> LFRAL;> AKCVSYGVAQIKAPALHSQGYTGSNVKVAILGTGIDSSHPDLNVAG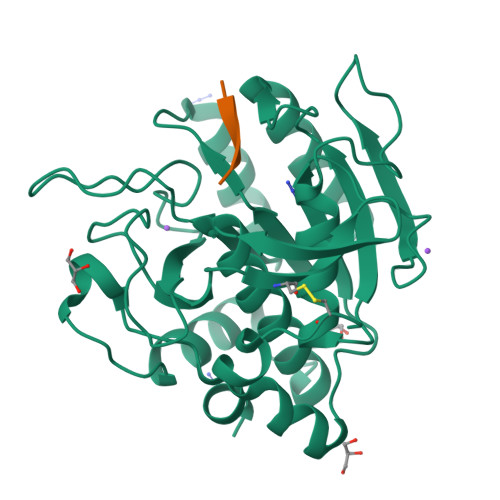GASFVPSETNPFQDNSSHGTHIAGTVLAVAPSASLYAVKVLGADGSGQASWVINGIEWAIANNMDVINMSLGSPSGSAALKAAVDKAVASGVVVVAAAGNSGTSGSSSTVTYPAKYPSVIAVGAVDSSNQRAPFSSVGPELDVMAPGVSICSTLPGGKYGALSGTSMASPHVAGAAALILSKHPNWTNTQVRSSLENTATKLGDSFYYGKGLINVEAAAQ> GSFNFNDEQYEEFINL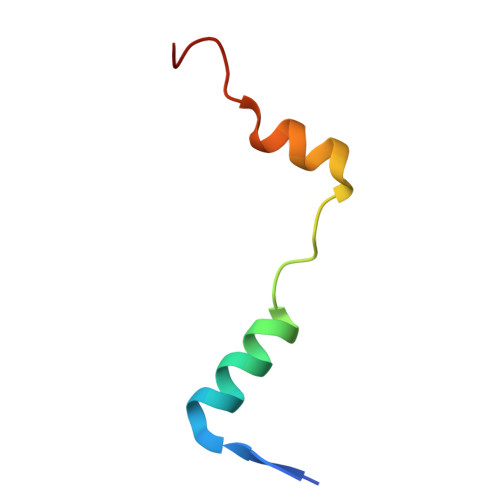LDAPVADDPVIEKLLARKPQWDV> GSMSGDPIRLRHLYTSGPHGLSSCFLRIRADGVVDCARGQSA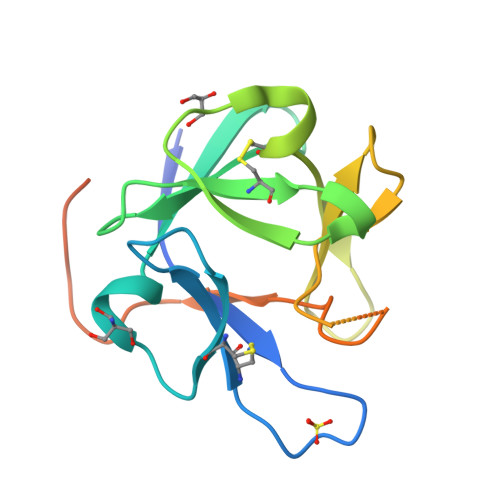HSLLEIKAVALRTVAIKGVHSVRYLCMGADGKMQGLLQYSEEDCAFEEEIRPDGYNVYRSEKHRLPVSLSSAKQRQLYKNRGFLPLSHFLPMLPMVPEEPEDLRGHLESDMFSSPLETDS> MQTDTSNRLKQIMAERNLKQVDILNLSIPFQKKFGIKLSKSTLSQYVNSVQSPDQNRIYLLAKTL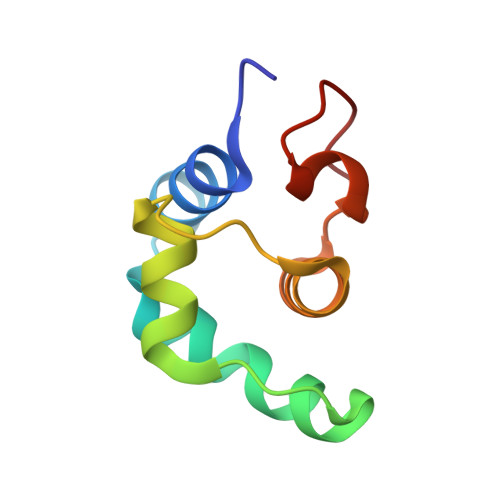GVSEAWLMGFDVPMV>MTQFEGFTNLYQVSKTLRFELIPQGKTLKHIQEQGFIEEDKARNDHYKELKPIIDRIYKTYADQCLQLVQLDWENLSAAIDSYRKEKTEETRNALIEEQATYRNAIHDYFIGRTDNLTDAINKRHAEIYKGLFKAELFNGKVLKQLGTVTTTEHENALLRSFDKFTTYFSGFYENRKNVFSAEDISTAIPHRIVQDNFPKFKENCHIFTRLITAVPSLREHFENVKKAIGIFVSTSIEEVFSFPFYNQLLTQTQIDLYNQLLGGISREAGTEKIKGLNEVLNLAIQKNDETAHIIASLPHRFIPLFKQILSDRNTLSFILEEFKSDEEVIQSFCKYKTLLRNENVLETAEALFNELNSIDLTHIFISHKKLETISSALCDHWDTLRNALYERRISELTGKITKSAKEKVQRSLKHEDINLQEIISAAGKELSEAFKQKTSEILSHAHAALDQPLPTTLKKQEEKEILKSQLDSLLGLYHLLDWFAVDESNEVDPEFSARLTGIKLEMEPSLSFYNKARNYATKKPYSVEKFKLNFQRPTLASGWDVNKEKNNGAILFVKNGLYYLGIMPKQKGRYKALSFEPTEKTSEGFDKMYYDYFPDAAKMIPKCSTQLKAVTAHFQTHTTPILLSNNFIEPLEITKEIYDLNNPEKEPKKFQTAYAKKTGDQKGYREALCKWIDFTRDFLSKYTKTTSIDLSSLRPSSQYKDLGEYYAELNPLLYHISFQRIAEKEIMDAVETGKLYLFQIYNKDFAKGHHGKPNLHTLYWTGLFSPENLAKTSIKLNGQAELFYRPKSRMKRMAHRLGEKMLNKKLKDQKTPIPDTLYQELYDYVNHRLSHDLSDEARALLPNVITKEVSHEIIKDRRFTSDKFLFHVPITLNYQAANSPSKFNQRVNAYLKEHPETPIIGIDRGERNLIYITVIDSTGKILEQRSLNTIQQFDYQKKLDNREKERVAARQAWSVVGTIKDLKQGYLSQVIHEIVDLMIHYQAVVVLENLNFGFKSKRTGIAEKAVYQQFEKMLIDKLNCLVLKDYPAEKVGGVLNPYQLTDQFTSFAKMGTQSGFLFYVPAPYTSKIDPLTGFVDPFVWKTIKNHESRKHFLEGFDFLHYDVKTGDFILHFKMNRNLS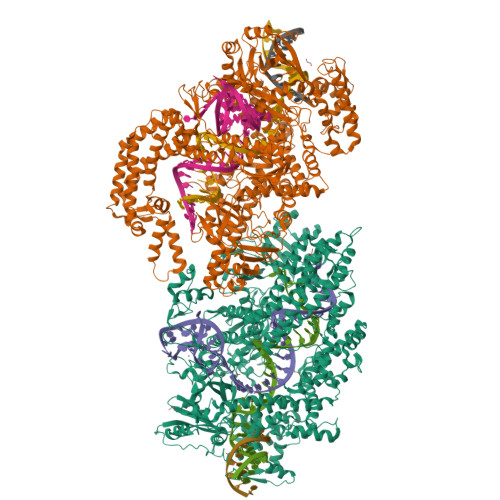FQRGLPGFMPAWDIVFEKNETQFDAKGTPFIAGKRIVPVIENHRFTGRYRDLYPANELIALLEEKGIVFRDGSNILPKLLENDDSHAIDTMVALIRSVLQMRNSNAATGEDYINSPVRDLNGVCFDSRFQNPEWPMDADANGAYHIALKGQLLLNHLKESKDLKLQNGISNQDWLAYIQELRN[2x]N-[3-(2,4-DICHLOROPHENOXY)PROPYL]-N-METHYL-N-PROP-2-YNYLAMINE | C13 H15 Cl2 N O | 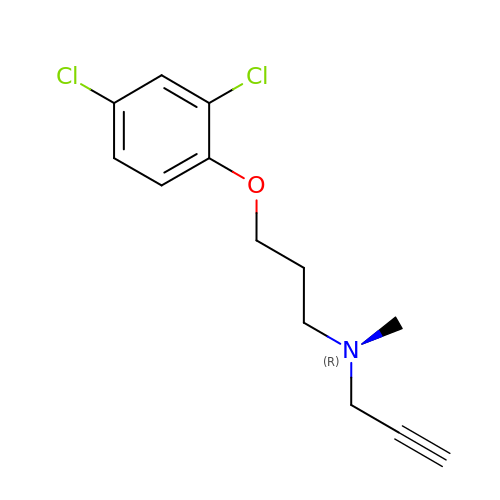BTFHLQRNAMSNLC-UHFFFAOYSA-N>MTQAKAKHADVPVNLYRPNAPFIGKVISNEPLVKEGGIGIVQHIKFDLTGGNLKYIEGQSIGIIPPGVDKNGKPEKLRLYSIASTRHGDDVDDKTISLCVRQLEYKHPESGETVYGVCSTYLTHIEPGSEVKITGPVGKEMLLPDDPEANVIMLATGTGIAPMRTYLWRMFKDAERAANPEYQFKGFSWLVFGVPTTPNILYKEELEEIQQKYPDNFRLTYAISREQKNPQGGRMYIQDRVAEHADQLWQLIKNQKTHTYICGLRGME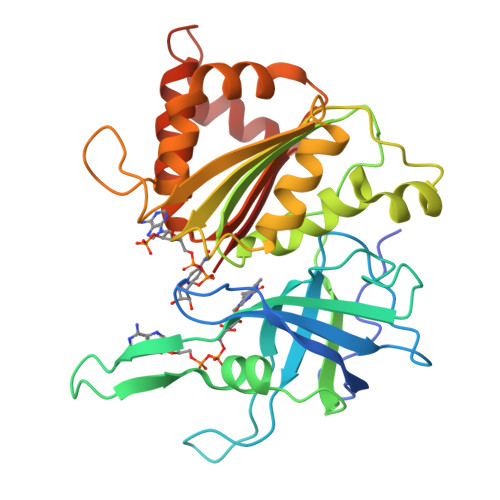EGIDAALSAAAAKEGVTWSDYQKDLKKAGRWHVETW[2x]>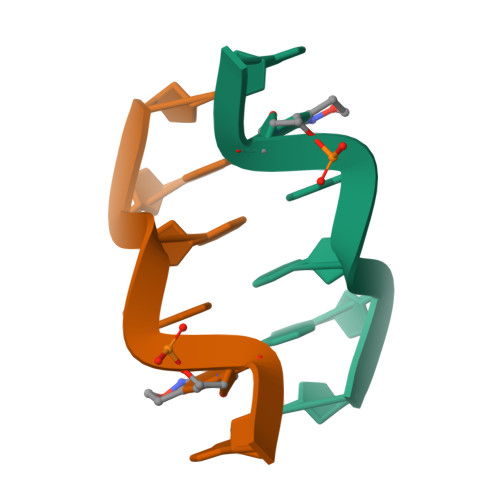CACGCG[2x]>MRDKFMDEFFKQVEEIRQYIDRIAENVEEVARQHQAILASPNPNWFDISQLLWLMADIKETANEVRKKLKEIEQSIEQEEGKNKSSADLKIRKRQHEELERKFREVMKEYNAT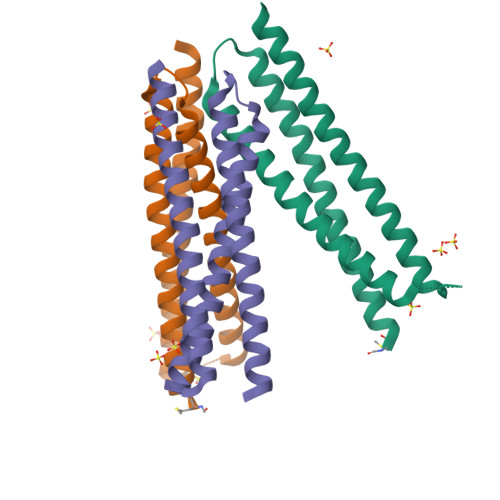QQDYRKRARKRNLEHHHHHH[3x]> ETGSLYLWIDAHQARVLIGFEEDILIVSEGKMAPFTHDFRKAQQRWPAIPVNIHSMNFTWQAAGQAEYFYEFLSLRSLDKGIMADPTVNVPLLGTVPHKASVVQVGFPCL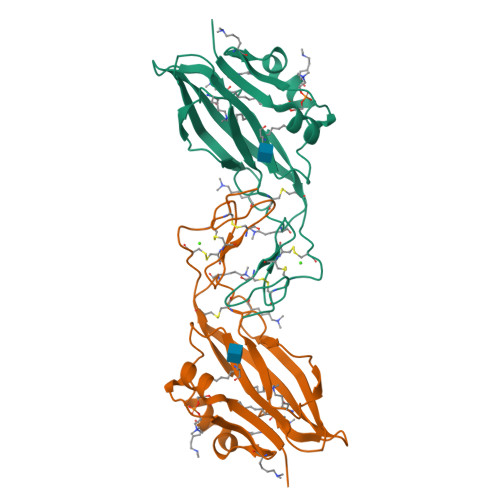GKQDGVAAFEVDVIVMNSEGNTILKTPQNAIFFKTCQQAECPGGCRNGGFCNERRICECPDGFHGPHCEGTKHHHHHH> MSMYTTAQLLAANEQKFKFDPLFLRLFFRESYPFTTEKVYLSQIPGLVNMALYVSPIVSGEVIRSRGGSTSEFTPGYVKPKH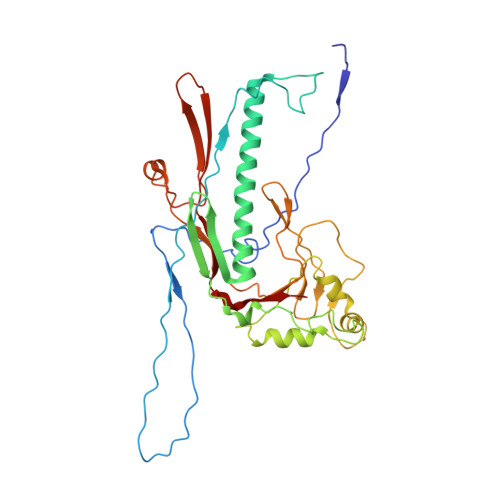EVNPQMTLRRLPDEDPQNLADPAYRRRRIIMQNMRDEELAIAQVEEMQAVSAVLKGKYTMTGEAFDPVEVDMGRSEENNITQSGGTEWSKRDKSTYDPTDDIEAYALNASGVVNIIVFDPKGWALFRSFKAVKEKLDTRRGSNSELETAVKDLGKAVSYKGMYGDVAIVVYSGQYVENGVKKNFLPDNTMVLGNTQARGLRTYGCIQDADAQREGINASARYPKNWVTTGDPAREFTMIQSAPLMLLADPDEFVSVQLA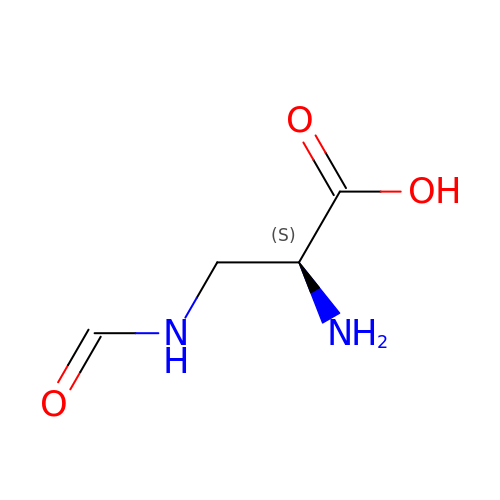3-(formylamino)-L-alanine | C4 H8 N2 O3 | VJGQHMAKHZCYRV-VKHMYHEASA-N> MSLKVVIGYLALDDWEFESLFPTIEWKYLTHINASFARVKADGTLNINPVRKRIESVRETAHKHNVKILISLAKNSPGEFTTAINDPKARKELIQQIIAFTKEYKLDGFDIDYEEYDNWDKNFPSLLVFARGLYLAKEKNMLMTCAVNSRWLNYGTEWEQYFDYINLMSYDRGAFTDKPVQHASYDDFVKDLKYWNEQCRASKSKIVGGLPFYGYSWEESLQGAVDDVRGIRYSGILKHLGNEAADKDNIGKTYYNGRPTIANKCKFIKENDYAGVMIWQLFQDAHNDNYDLK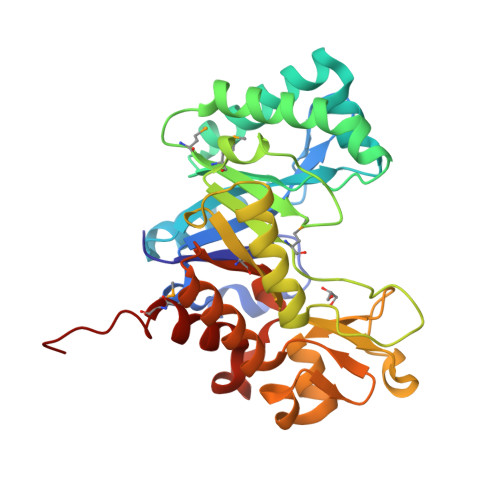LINVVGREMMEEGHHHHHH>MKQTVAAYIAKTLESAGVKRIWGVTGDSLNGLSDSLNRMGTIEWMSTRHEEVAAFAAGAEAQLSGELAVCAGSCGPGNLHLINGLFDCHRNHVPVLAIAAHIPSSEIGSGYFQETHPQELFRECSHYCELVSSPEQIPQVLAIAMRKAVLNRGVSVVVLPGDVALKPAPEGATMHWYHAPQPVVTPEEEELRKLAQLLRYSSNIALMCGSGCAGAHKELVEFAGKIKAPIVHALRGKEHVEYDNPYDVGMTGLIGFSSGFHTMMNADTLVLLGTQFPYRAFYPTDAKII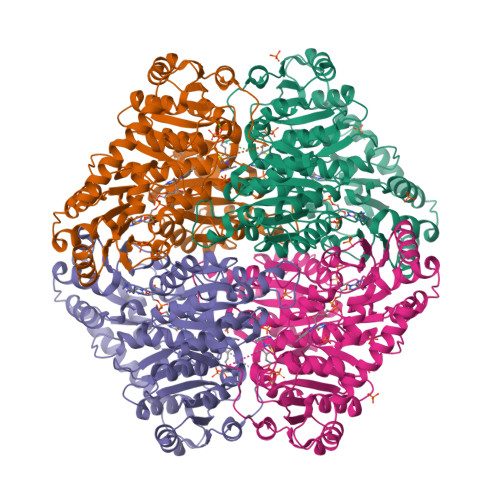QIDINPASIGAHSKVDMALVGDIKSTLRALLPLVEEKADRKFLDKALEDYRDARKGLDDLAKPSEKAIHPQYLAQQISHFAADDAIFTCDVGTPTVWAARYLKMNGKRRLLGSFNHGSMANAMPQALGAQATEPERQVVAMCGDGGFSMLMGDFLSVVQMKLPVKIVVFNNSVLGFVAMEMKAGGYLTDGTELHDTNFARIAEACGITGIRVEKASEVDEALQRAFSIDGPVLVDVVVAKEELAIPPQIKLEQAKGFSLY[12x]> SANEDMPVEKILEAELAVEPKTETYVEANMGLNPSSPNDPVTNICQAADKQLFTLVEWAKRIPHFSELPLDDQVILLRAGWNELLIASASHRSIAVKDGILLATGLHVHRNSAHSAGVGAIFDRVLTELVSKMRDMQMDKTELGCLRAIVLFNPDSKGLSNPAEVEALREKVYASLEAYCKHKYPEQPGRFAKLLLRLPALRSIGLKCLEHLFFFKLIGDTPIDTFLMEML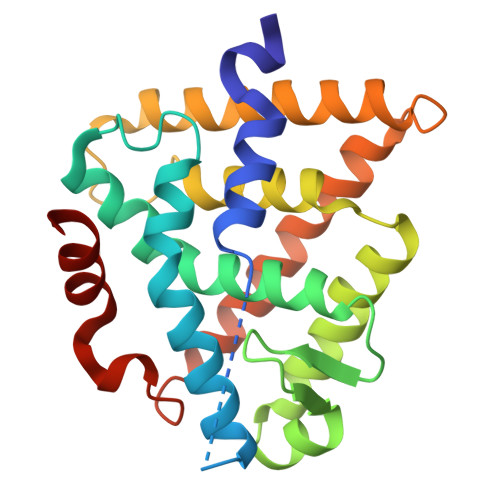EA> GPPDLGTDDDDKAMADIASCTTQEKTAPVISVAEQAVPSISEIDRSYLLSSDRLTEVDGNTLDVASEEQVAALKAQFENLKDGDEVVIPNGKYANLGQVTITANDVTIRAEQAGAAWLTGLIQFELKGDDITLDGLVFTEGGPNERFGA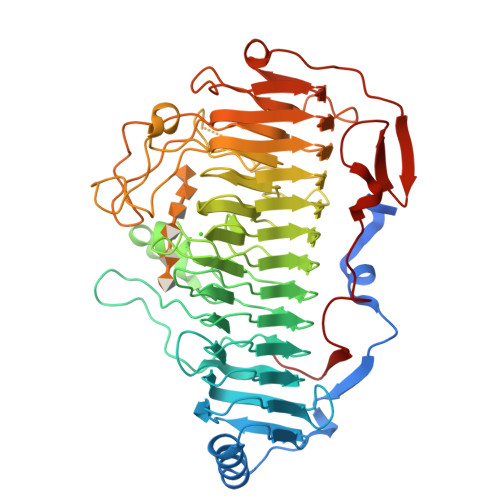VRMMGNGNTLQNSTFYYFNHDYTYEPDERRSEYPKYLWVSLWGKDGKVINNRFEGKQKRGTLIGVQKDDTPDNHLIANNIFMDQKPNQFNEFDIKEAIRYNGNSWEAIRIGDSKSSQWDSSSKFVNNLMIDMDGERELISIASGDNTISGNTIFQSAALISLRHGKGNTVENNMILGNEKRLTGGIRIYDEDHVIRNNYIANTRGRDGVIEGNADLRGGIVINTGIIDVANGEQLDQSVKGKELNKQWTPKNITIENNSLVDTEWGIVYGNQSHRVSLFNNAEVEGIYAGVDIAFKHNVVDNSQTPEFVSVRATHDFPLVGATYTDETYVGQVTDSELIESYSVELPKVTVENGLNAYQGEGADVSKLSVVTAETAGPDYVLENTTK> VYVPDEWEVAREKITMSRELGQGSFGMVYEGVAKGVVKDEPETRVAIKTVNEAASMRERIEFLNEASVMKEFNCHHVVRLLGVVSQGQPTLVIMELMTRGDLKSYLRSLRPEMENNPVLAPPSLSKMIQMAGEIADGMAYLNANKFVHRDLAARNCMVAEDFTVKIGDFGMTRDIYETDYYRKGGKGLLPVRWMSPESLKDGVFTTYSDVWSFGVVLWEIATLAEQPYQGLSNEQVLRFVMEGGLLDK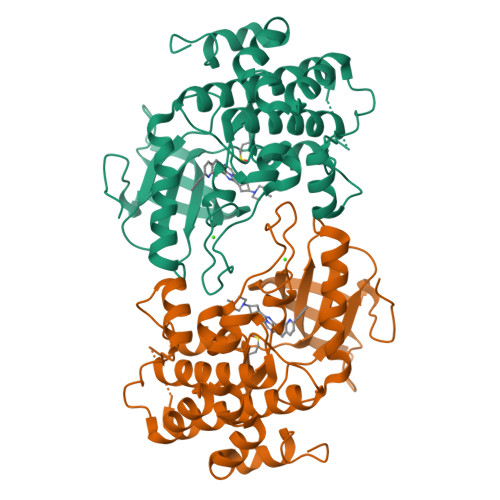PDNCPDMLLELMRMCWQYNPKMRPSFLEIISSIKEEMEPGFREVSFYYSEENK> MQQQTLPKPFIWAEPHFMVPKEKQVTICCQGNYGAVEYQLHFEGSLFAVDRPKPPERINKVKFYIPDMNSRMAGQYSCIYRVGELWSEPSNLLDLVVTEMYDTPTLSVHPGPEVISGEKVTFYCRLDTATSMFLLLKEGRSSHVQRGYGKVQAEFPLGPVTTAHRGTYRCFGSYNNHAWSFPSEPVKLLVTGDLEHHHHHH;> ACY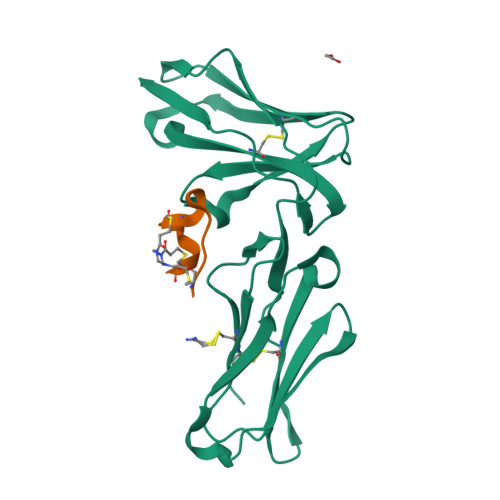XPDYLCADEYCAX>MGKSLSHLPLHSSKEDAYDGVTSENMRNGLVNSEVHNEDGRNGDVSQFPY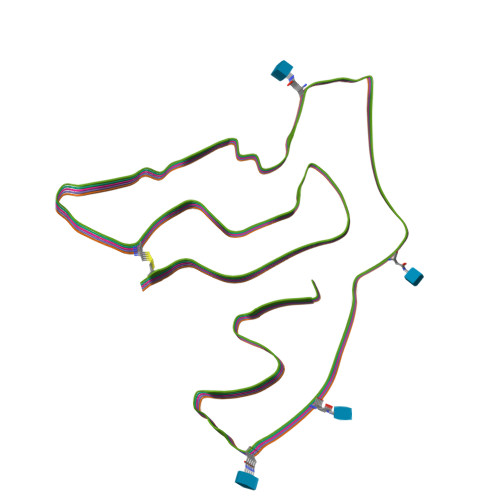VEFTGRDSVTCPTCQGTGRIPRGQENQLVALIPYSDQRLRPRRTKLYVMASVFVCLLLSGLAVFFLFPRSIDVKYIGVKSAYVSYDVQKRTIYLNITNTLNITNNNYYSVEVENITAQVQFSKTVIGKARLNNITIIGPLDMKQIDYTVPTVIAEEMSYMYDFCTLISIKVHNIVLMMQVTVTTTYFGHSEQISQERYQYVDCGRNTTYQLGQSEYLNVLQPQQ[5x]>MKSNGCRYGTHRVIEPKGVLPQPAKILNNDMSEIWDNEMLIDVIRLNIDSASFHQIKNKLIAQGHQDLEKAFAEHAIELTNRTGKHKNEDTGSGGMFIGRVAAIGDKFEMKEEVKVGDKIASLVSLSLTPLKINKVKKV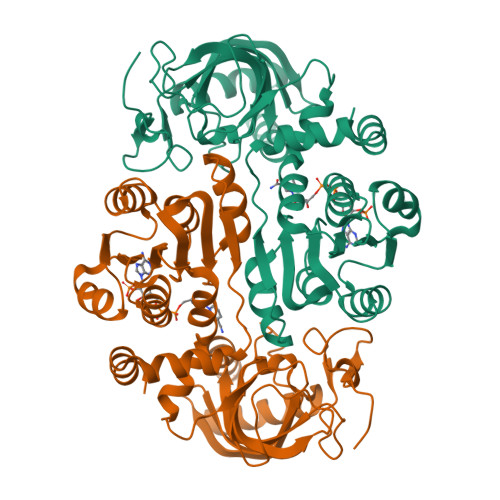LLDKDQMEIEGQAILFSSGVYAKLPDDLDENLALSVLDVAGAPAQVERLVKPDDTVVIIGANGKSGILCNAVAKERAGICGKVIGVVRNENYIPTCKATGCDEVILAQATDAITIQKEVSRLTNGKMADVVINVVNTEDTELPSIMAAKDRGMVYFFSMATSFTKAALGAGGIGADVDMMIGNSYAHHHSEIALDLLRRNSVLMKIFKERYAEHHHHHH[4x]N-(6-chloro-3,3-dimethyl-3,4-dihydroisoquinolin-1-yl)-3-(4-propylthiophen-3-yl)-L-alanine | C21 H25 Cl N2 O2 S | 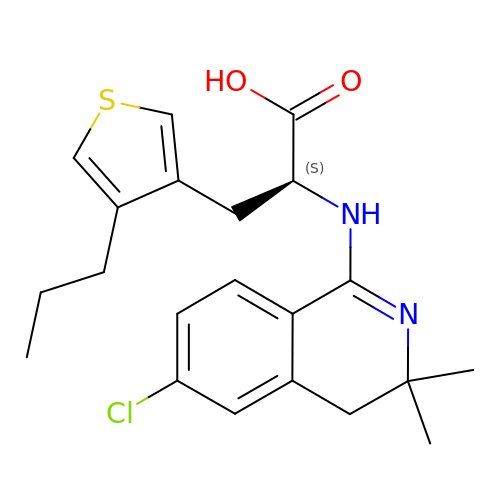SFUUSYIYAKSHRW-SFHVURJKSA-N>[3x]NDKLIELSNSNENWVMPGKNYDSNNYSTSTQINVDNVKQLKHAWSFSTGELHGHEGAPLVIGDVMYVHSSFPNKTFALDLNDPGHILWQHSPKQDPAARSVACCDLVNRGLAYWPGDDKTPSLIIKTQLDGHLVALNAKTGEEFWKVENGDIKVGQTLTQAPYVVHDLAIVGSSGAELGVRGHVTAYNVRTGEQAWRYYATGPDAEIGLADDFNSANPHYGQKGLGTATWEGDAWKIGG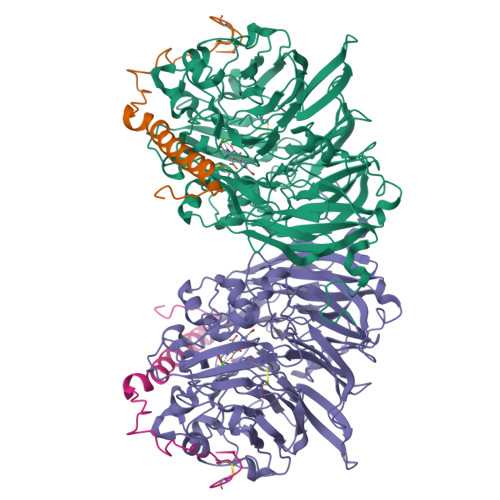GTNWGWYAYDPAANLIYYGSGNPAPWNETMRPGDNKWTMTITARDADTGKMKFGYQKTPHDEWDFAGVNVIMLSEQTDKTGKKRKLLTHPDRNGIVYTLDRENGDLISADKLDDTVNVFKTVDLKTGLPVRDPEYGTRMDHKGTDICPSAMGYHNQGHDSYDPQKQLFFMGINHICMDWEPFMLPYRAGQFFVGATLWMYPGPKGDRQNYLGLGQIKAYNAITNEYKWQHMERFSVWGGTLATAGNLVFYGTLDGFLKARNSDTGELVWKHKLPSGVIGYPMTYEHKGVQYIAVMSGVGGWPGVGLVFDLQDPTAGLGAVGAFKNLQNYTQMGGSLEVFSLDGKNPYDDVNVGEYEKG;>YDGTHCKAPGNCWEPKPGFPEKIAGSKYDPKHDPKELNKQVESRKGEEERNANRAEHFKKTGKWVYDVKKIQ[3x]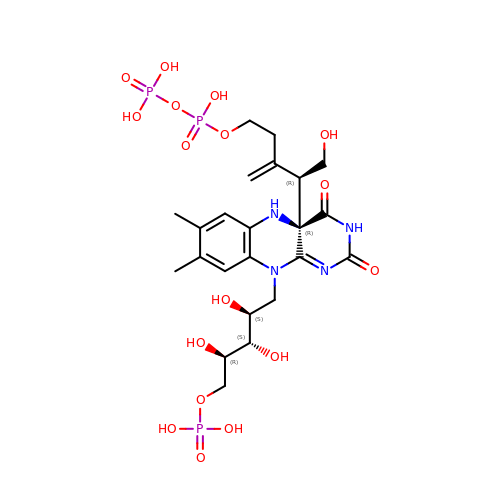1-deoxy-1-[(4aR)-4a-[(2R)-1-hydroxy-5-{[(S)-hydroxy(phosphonooxy)phosphoryl]oxy}-3-methylidenepentan-2-yl]-7,8-dimethyl-2,4-dioxo-3,4,4a,5-tetrahydrobenzo[g]pteridin-10(2H)-yl]-5-O-phosphono-D-ribitol | C23 H35 N4 O17 P3 | KSKIGIXASYOSHG-TUUFUFLPSA-N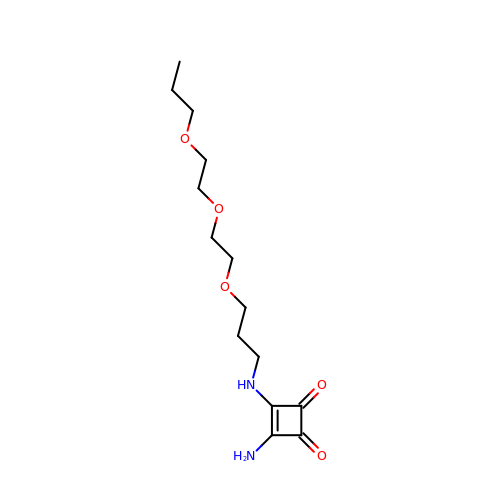3-AMINO-4-{3-[2-(2-PROPOXY-ETHOXY)-ETHOXY]-PROPYLAMINO}-CYCLOBUT-3-ENE-1,2-DIONE | C14 H24 N2 O5 | ZUVPNXOKAPTNLU-UHFFFAOYSA-N> ATHIAIC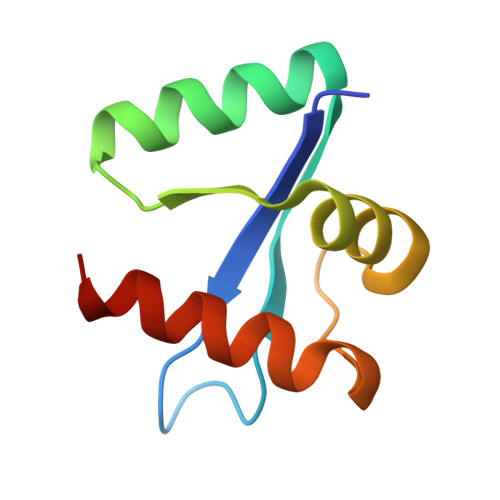LYYKLGETPLPLVIETGKDAKALQIIKLAELYDIPVIEDIPLARSLYKNIHKGQYITEDFFEPVAQLIRIAIDLDY>MRFLKRKKSLSAGMLLALAVGSAASIPSAYSNDDVLKLTENPKNWAAPGKDYANTRHSPLKQINTQNVKGLHMAWSFSTGVLRGHEGQPLVIGDRMYVVTPYPNIVWALDISKGNSYEVLWKYAPRQDDKAVSTACCDTVNRGASYADGKIVFNTLDGYVVCLDANTGKELWKTKFADVNKGETSTPAPIIVKDKVVTGYGGDEFGARGRFAAFDLNSGKMVWQAYSNGPDSDVLLGPDFNSKHPEYGQAGQDLGVKTYPDEEWKRGGGCAWGWYSYDPKLDLIYYNTGNPGLWSPSYRTEAKTHEEANEPWKWDNKWSMTIFARKPDTGEAVWGYQMTPFDQWDYDGINEDVLVDITVDGSKKPCLVHFDRNGFCYVLNRTDGTIIRANKFVTVNWAEKIDMKTGRPVKVKEHSPFEVGKAVQAYPSAMGGKDQQPVAVDPKEPNVFYAPTNNWGMTLEPMERAHTNQGSVYVFANVLMKPEKPGVMGRFKAFDVITGKARWDIPERFPTWSGALVTDGGLAFYGTLDGWFKAVDRKTGKVLWQQKLGSGIIGNPISYEVGGKQYISVLSGIGGWIGLPVTAGLDPADPYGALGVSGMAAENGFYNIPMGGTLYTFCVQ[2x]

Remarkably, the same elements are actively taken up by methanotrophs/methylotrophs in a range of environments, since their XoxF-type methanol dehydrogenases require lanthanides as a metal cofactor. Interestingly, XoxF does not form a complex with a small subunit, but forms a homodimer. Here, we report the purification and characterization of the XoxF1-type MDH from the acidophilic methanotroph Methylacidimicrobium thermophilum AP8.

By cultivating M. thermophilum AP8 in medium supplemented with 0.5 μM Nd2O3 as the sole lanthanide at μmax (0.051 h−1) on methane, we aimed to study a functional neodymium-containing methanol dehydrogenase enzyme and determine the structure of the catalytic site. The crystal structure of Nd-XoxF1 contains a dimer in the asymmetric unit, of which one monomer contains no PQQ molecule and the other contains a PQQ molecule and neodymium ion with approximately 70% occupancy. The loss of the PQQ cofactor from the enzyme is interesting and could be a combined result of the exchange of buffers and the high salt concentration used during the crystallization procedure. The two monomers show the typical eight-bladed β-propeller fold of a methanol dehydrogenase, a conserved disulfide bridge above the PQQ cofactor and an aspartate residue coordinating the lanthanide in the active site. They can be superimposed with the structure of the cerium-containing XoxF2 of Methylacidiphilum fumariolicum SolV to a root mean square deviation (RMSD) of 0.8 Å. However, a detailed comparison of the Nd-XoxF1 structure with those of other XoxF-type and MxaFI-type MDHs reveals an interesting difference in the direct vicinity of the active site, namely, position 172, which directly precedes the Nd-coordinating Glu173, is occupied by an aspartate residue in Nd-XoxF1, whereas this residue is a glycine in all other known MDH structures. Amino acid sequence alignments of a large variety of methanol and alcohol dehydrogenases reveals that the presence of an aspartate residue in this position is diagnostic for the XoxF1 lineage. To accommodate the Asp172 side chain, residue 240 is a cysteine in Nd-XoxF1, whereas it is a bulkier threonine in XoxF2 of M. fumariolicum SolV. With respect to the XoxF2 structures of Methylacidiphilum fumariolicum SolV, the presence of Asp172 (replacing glycine) results in a rearrangement of the loop containing the metal-coordinating Glu173. The coordination of PQQ and the lanthanide are almost identical to the coordination in other XoxF-type MDHs, and therefore the overall coordination of the lanthanide is not altered in XoxF1 compared to that of other XoxF-type MDHs.> MKKVIIAGNGPSLKEIDYSRLPNDFDVFRCNQFYFEDKYYLGKKCKAVFYNPSLFFEQYYTLKHLIQNQEYETELIMCSNYNQAHLENENFVKTFYDYFPDAHLGYDFFKQLKDFNAYFKFHEIQFNQRITSGVYMCAVAIALGYKEIYLSGIDFYQNGSSYAFDTKQKNLLKLAPNFKNDNSHYIGHSKNTDIKALEFLEKTYKIKLYCLCPNSLLANFIGL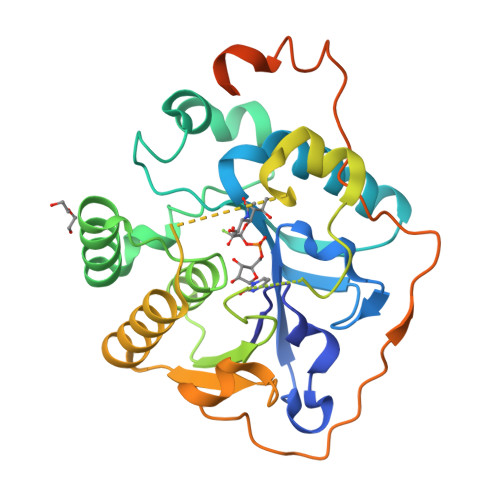APNLNSNFIIQEKNNYTKDILIPSSEAYGKFSKNINFKKIKIKENIYYKLIKDLLRLPSDIKHYFKGK methyl [(2R,7S)-7-({(2E)-3-[5-chloro-2-(1H-tetrazol-1-yl)phenyl]prop-2-enoyl}amino)-2-(trifluoromethyl)-2,3,4,5,6,7-hexahydro-1H-8,11-epimino-1,9-benzodiazacyclotridecin-14-yl]carbamate 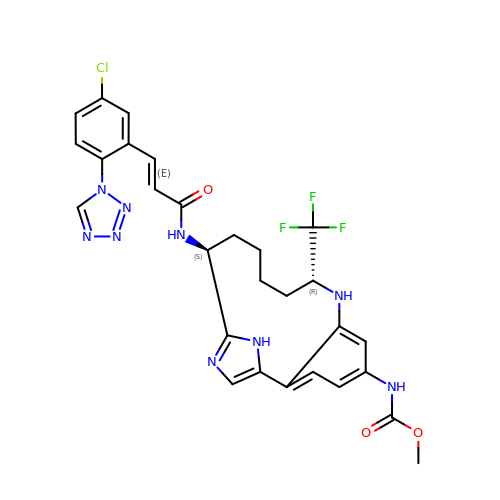| C28 H27 Cl F3 N9 O3 | UXHSEEJCQYWDBB-UENHJXRBSA-N> MRGSHHHHHHGSACELGTPNMSEEVSKNLSETLFVKHKQAKETSALTQYMPTSQSLLDEIKEKNGFSWYRNLRRLQWVWQGVDPIEQEQVLARIASSKHSRTDEQWLDTVMGYHSGNWAYEWTRLGMEHQKRAGEMTNEAASEALFSASLCYSIAGYPHLKSDNLAIQAQVLANSAYLEAAKKSKYIIKQLEIPFEKGKITAHLHLTNTDKPHPVVIVSAGLDSLQTDMWRLFRDHLAKHDIAMLTVDMPSVGYSSKYPLTEDYSRLHQAVLNELFSIPYVDHHRVGLIGFRFGGNAMVRLSFLEQEKIKACVILGAPIHDIFASPQKLQQMPKMYLDVLASRLGKSVVDIYSLSGQMAAWSLKVQGFLS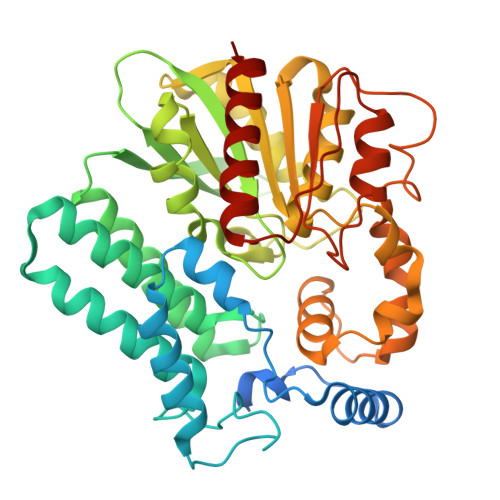SRKTKVPILAMSLEGDPVSPYSDNQMVAFFSTYGKAKKISSKTITQGYEQSLDLAIKWLEDELLR>[3x]MRGSHHHHHHGSSAVSTTAAPEARSILAGAAEGKVIATTEALSFWGGVDPATGKVIDVHHPLHGICLTGGVLFMPTSRGSCTGSGVLLDLILTGRAPSALVFCEAEDVLTLGALVAAEMFDKALPVIRLDTETFARFSRAAHVRIDQNTIKADGVSLAVAPPATAHLDLTDDDRAMLEGRDGIAVRQAMRIIVAMAAQQGASALVDVTQGHIDGCIYASPANLTFAEKMADMGGKVRVPSTMNAISVDKANWRAQGVPEDFGDPAARLADAYVRMGCRPTFTCSPYLLDSAPSAGESIGWAESNAVIFANTVLGARTAKHPDFLDLCIAMTGRAPLSGVYLEENRRPQRIVDVALPAGIDDAFWPLVGYLAGKAVPDCIPLLRGLGAAKPSRDDLKALCAAFGTTSASPMLHIEGATPEAGLAPLETAETVTISLEDMAAGWSLLNEGPEEVQLVAIGSPHASLEECRALAAVFNGRKRHADVAVIVTAGQQVIDAAGKDGTLQSLKDSGVQVLPDLCWCSISEPVFPTKTRALMTNSGKYAHYGPGLSGRAVRFGSLADCVESALTGRAVSRLPVWLS

Aconitase superfamily members catalyze the homologous isomerization of specific substrates by sequential dehydration and hydration and contain a [4Fe-4S] cluster. However, monomeric and heterodimeric types of function unknown aconitase X (AcnX) have recently been characterized as a cis-3-hydroxy-L-proline dehydratase (AcnXType-I) and mevalonate 5-phosphate dehydratase (AcnXType-II), respectively. We herein elucidated the crystal structures of AcnXType-I from Agrobacterium tumefaciens (AtAcnX) and AcnXType-II from Thermococcus kodakarensis (TkAcnX) without a ligand and in complex with substrates. AtAcnX and TkAcnX contained the [2Fe-2S] and [3Fe-4S] clusters, respectively, conforming to UV and EPR spectroscopy analyses.

The crystal structure was elucidated by the single-wavelength anomalous dispersion (SAD) method using the selenomethionine (SeMet)-substituted crystal, and subsequently refined to a resolution of 1.6 Å against the data set from the native crystal. The three molecules in the asymmetric unit were essentially identical, being superimposable with a root-mean-square deviation (r.m.s.d.) of 0.4–0.7 Å over 552–558 Cα atoms. Alternatively, we attempted to separately superimpose each domain of mAcn onto the crystal structure of AtAcnX, and found that domains 1–4 of AtAcnX each consisted of 157–336, 337–435, 436–569, and 1–149 residues in the order of 4-1-2-3, respectively, from the N to C terminus. AtAcnX crystals were brown in color, similar to the purified protein, strongly indicating the maintenance of cofactors. The electron density map suggested that this enzyme had a planar [2Fe-2S] cluster (gray mesh in Fig. 4a) located within a solvent-filled cleft in the protein structure. Fe2 and Fe1 atoms were tetrahedrally coordinated by two bridging sulfide ions and two cysteine residues (Cys273 and Cys508) and by two bridging sulfide ions, one water molecule, and one cysteine (Cys510), respectively. The water molecule further formed hydrogen bonds with the side chains of Glu292 and Lys530. The superpositions of the overall crystal structures showed that the [2Fe-2S] cluster in AtAcnX was roughly located at a similar position to the [4Fe-4S] cluster in mAcn. Among the [Fe-S] cluster-binding sites, only two adjacent Cys508 (green) and Cys510 (blue) in AtAcnX were located at equivalent (or close) positions to Cys421 and Cys424 in mAcn; the characteristic motifs of Cys-X-Cys and Cys-X-X-Cys were often detected in other [Fe-S] cluster-containing proteins. On the other hand, AtAcnX possessed Cys273 (yellow-green) at an equivalent position to His147 in mAcn, whereas no homologous cysteine residues to Cys358 were found in mAcn.>[2x]GSMRDKLLDFIIELSQ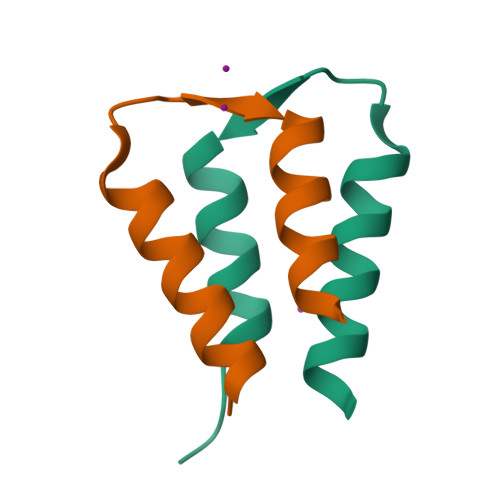SSKQVVSKSYVIDRLMQVTKEDYKELEKNVEGKKDD>GKLPPYIFSPIPFLGHAIAFGKSPIEFLENAYEKYGPVFSFTMVGKTFTYLLGSDAAALLFNSKNEDLNAEDVYSRLTTPVFGKGVAYDVPNPVFLEQKKMLKSGLNIAHFKQHVSIIEKETKEYFESWGESGEKNVFEALSELIILTASHCLHGKEIRSQLNEKVAQLYADLDGGFSHAAWLLPGWLPLPSFRRRDRAHREIKDIFYKAIQKRRQSQEKIDDILQTLLDATYKDGRPLTDDEVAGMLIGLLLAGQHTSSTTSAWMGFFLARDKTLQKKCYLEQKTVCGENLPPLTYDQLKDLNLLDRC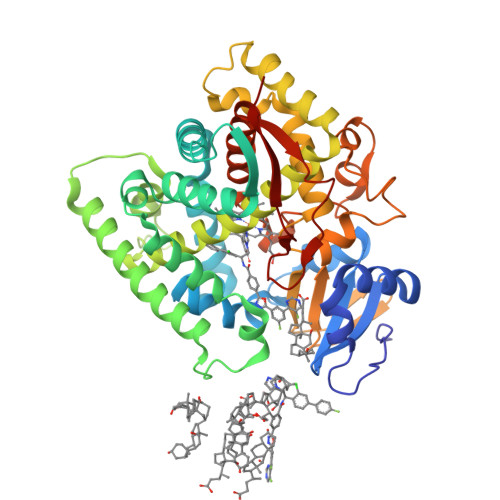IKETLRLRPPIMIMMRMARTPQTVAGYTIPPGHQVCVSPTVNQRLKDSWVERLDFNPDRYLQDNPASGEKFAYVPFGAGRHRCIGENFAYVQIKTIWSTMLRLYEFDLIDGYFPTVNYTTMIHTPENPVIRYKRRSK[2x]>[24x]PHFLILNGPNV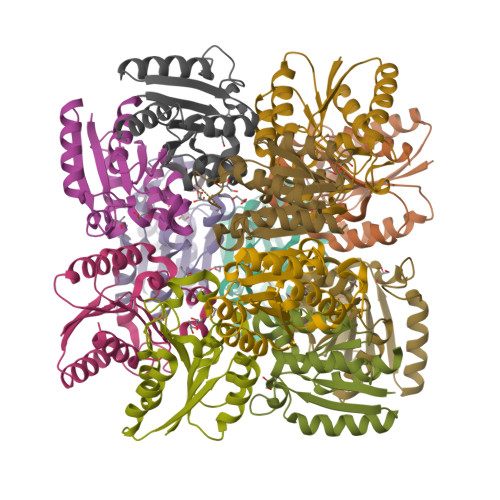NRLGSREPEVFGRQTLTDIETDLFQFAEALHIQLTFFQSNHEGDLIDAIHEAEEQYSGIVLNPGALSHYSYAIRDAVSSISLPVVEVHLSNLYAREEFRHQSVIAPVAKGQIVGLGAEGYKLAVRYLLSQQG> MRGSHHHHHHGSACELGTGLSIGIVGATGQVGQVMRTLLDERDFPASAVRFFASARSQGRKLAFRGQEIEVEDAETADPSGLDIALFSAGSAMSKVQAPRFAAAGVTV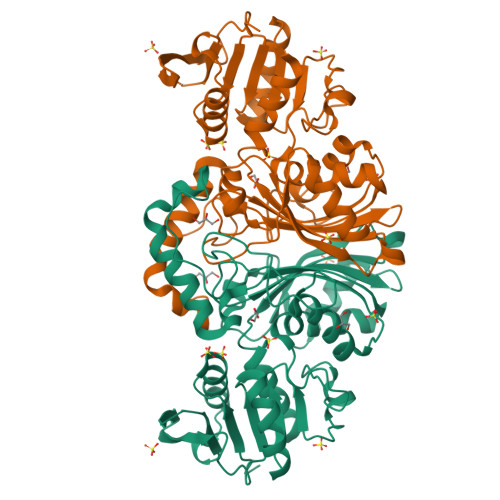IDNSSAWRKDPDVPLVVSEVNFERDAHRRPKGIIANPNCTTMAAMPVLKVLHDEARLVRLVVSSYQAVSGSGLAGVAELAEQARAVIGGAEQLVYDGGALEFPPPNTYVAPIAFNVVPLAGSLVDDGSGETDEDQKLRFESRKILGIPDLLVSGTCVRVPVFTGHSLSINAEFAQPLSPERARELLDGATGVQLVDVPTPLAAAGVDESLVGRIRRDPGVPDGRGLALFVSGDNLRKGAALNTIQIAELLTADL>[2x]MGSSHHHHHHSQDPLVPRGSHMLDPRLSVAPMVDRTDRHFRFLVRQVSLGVRLYTEMTVDQAVLRGNRERLLAFRPEEHPIALQLAGSDP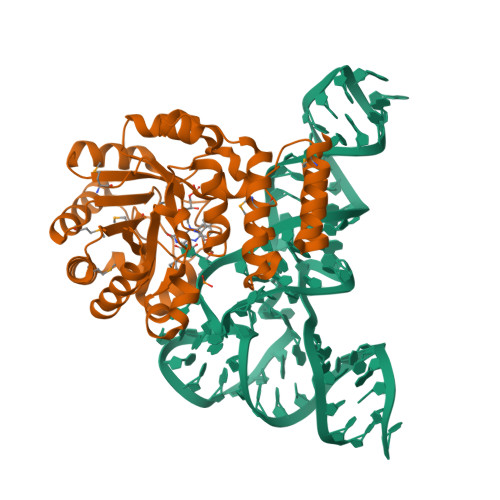KSLAEAARIGEAFGYDEINLNLGCPSEKAQEGGYGACLLLDLARVREILKAMGEAVRVPVTVKMRLGLEGKETYRGLAQSVEAMAEAGVKVFVVHARSALLALSTKANREIPPLRHDWVHRLKGDFPQLTFVTNGGIRSLEEALFHLKRVDGVMLGRAVYEDPFVLEEADRRVFGLPRRPSRLEVARRMRAYLEEEVLKGTPPWAVLRHMLNLFRGRPKGRLWRRLLSEGRSLQALDRALRLMEEEVGEEGEKEKPGPRGQREAAPGPAREGV7-hydroxy-3-(4-hydroxyphenyl)-4H-chromen-4-one 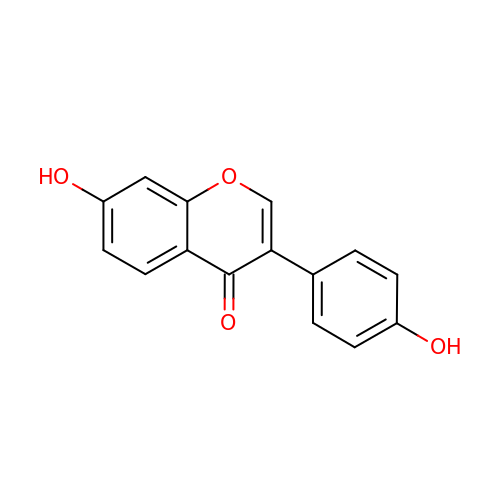| C15 H10 O4 | ZQSIJRDFPHDXIC-UHFFFAOYSA-N>TGDSEFCDMLRLFDFNKNAIEKLNNQTKTAVNMLTHSINSLISDNLLMRNKLKEVLKVPYCNYTRFWYINHTKSGEHSLPRCWLVSNGS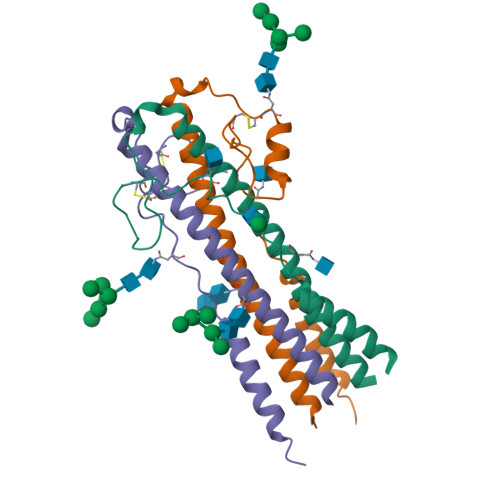YLNESDFRNEWILESDHLIAEMLSKEYQDRQGKTPLTLVDGTKHHHHHH[3x]> MAHHHHHHVGTGSNDDDDKSPDPWELTILHTNDVHSRLEQTSEDSSKCVDASRCMGGVARLFTKVQQIRRAEPNVLLLDAGDQYQGTIWFTVYKGAEVAHFMNALRYDAMALGNHEFDNGVEGLIEPLLKEAKFPILSANISASGPLASQISGLYLPYKVLPVGDEVVGIVGYTSKETPFLSNPGTNLVFEDEITALQPEVDKLKTLNVNKIIALGHSGFEMDKLIAQKVRGVDVVVGGHSNTFLYTGNPPSKEVPAGKYPFIVTSDDGRKVPVVQAYAFGKYLGYLKIEFDERGNVISSHGNPILLDSSIPEDPSIKADINKWRIKLDDYSTQELGKTIVYLDGSSQSCRFRECNMGNLICDAMINNNLRHADEMFWNHVSMCILNGGGIRSPIDERNDG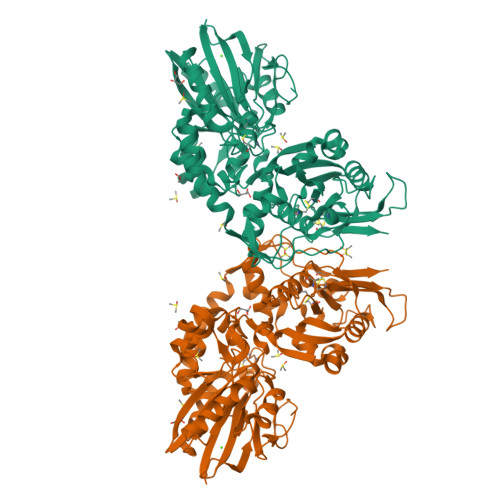TITWENLAAVLPFGGTFDLVQLKGSTLKKAFEHSVHRYGQSTGEFLQVGGIHVVYDLSRKPGDRVVKLDVLCTSCRVPSYDPLKMDEVYKVILPNFLANGGDGFQMIKDELLRHDSGDQDINVVSTYISKMKVIYPAVEGRIKFS>SFVEMVDNLRGKSGQGYYVEMTVGSPPQTLNILVDTGSSNFAVGAAPHPFLHRYYQRQLSSTYRDLRKGVYVPYTQGKWEGELGTDLVSIPHGPQVTVRANIAAITESDKFFIQGSNWEGILGLAYAEIARPDDSLEPFFDSLVKQTHVPNLFSLQLCGAGFPLQQSEVLASVGGSMIIGGIDHSLYTGSLWYTPIRREWYYEVIIVRVEINGQDLKMDCKEYNYDKSIVDSGTTNLRLPKKVFEAAVKSIKAASSTEKFPDGFWLGEQLVCWQAGTTPWNIFPVISLYLMGEVTQQSFRITILPQQYLRPVEDVATSQDDCYKFAISQSSTGTVMGAVIMEGFYVVFDRARK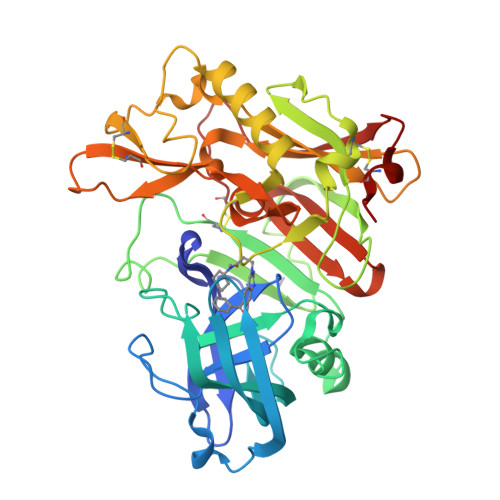RIGFAVSACHVHDEFRTAAVEGPFVTLDMEDCGYN[3x]>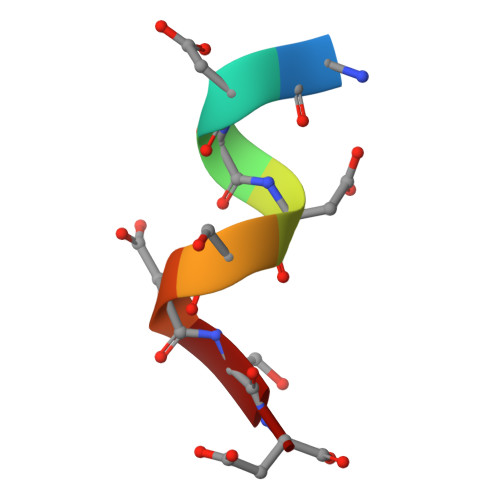 SDSDSDSD> MQPDTHLTDMLQQLAVVNAAKPSDRGFIRQEEAEDPACIPVFWISKWVDYSDKYGLGYQ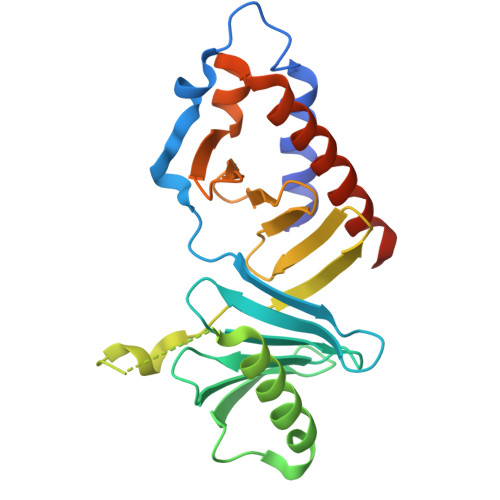LSDNSVGVLFNDSTRLIMCADGDSLQYIDRNSLESYLSVRSYPSALSKKITLLKYFRNYMSEHLLKAGANITPREGDELTRLPYLRHWFRTKSAIVLHLSNGTVQINFFQDHTKLILCPLMGAVTYINEKREFYTYKMTLIEEFGCCKELASRLRYARNMVEKLMACKSSTTAATSAR>[2x]MGNKEKA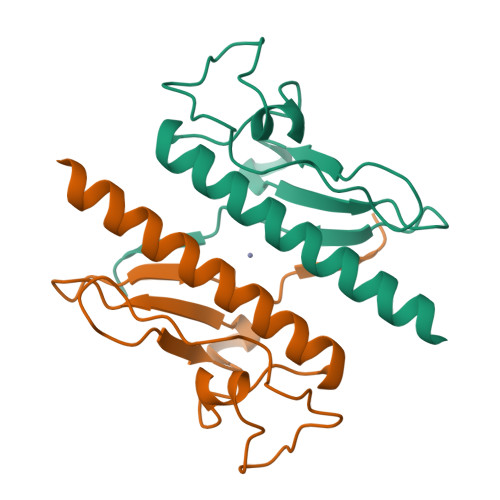DRQKVVSDLVALEGALDMYKLDNSRYPTTEQGLQALVSAPSAEPHARNYPEGGYIRRLPQDPWGSDYQLLSPGQHGQVDIFSLGPDGVPESNDDIGNWTIGFHHHHHHK> MEHVAFGSEDIENTLAKMDDGQLDGLAFGAIQLDGDGNILQYNA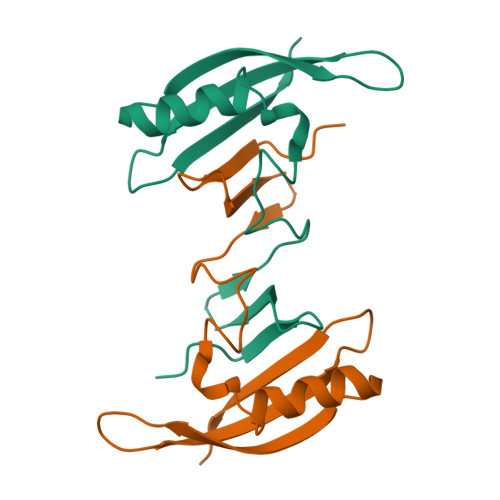AEGDITGRDPKQVIGKNFFKDVAPGTDSPEFYGKFKEGVASGNLNTMFEWMIPTSRGPTKVKVHMKKALSGDSYWVFVKRVKLAAALEHHHHHH> GRTNLIVNYLPQNMTQDELRSLFSSIGEVESAKLIRDKVAGHSLGYGFVNYVTAKDAERAINTLNGLRLQSKTIKVSYARPSSEVIKDANLYISGLPRTMTQKDVEDMFSRFGRIINS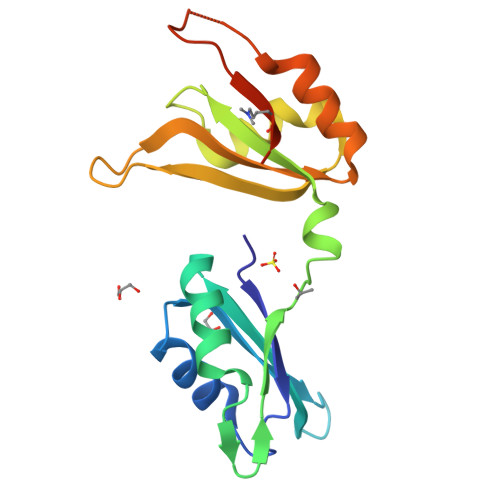RVLVDQTTGLSRGVAFIRFDKRSEAEEAITSFNGHKPPGSSEPITVKFAANLEHHHHHH>[4x]GSKLQICVEPTSQKLMPGSTLVLQCVAVGSPIPHYQWFKNELPLTHET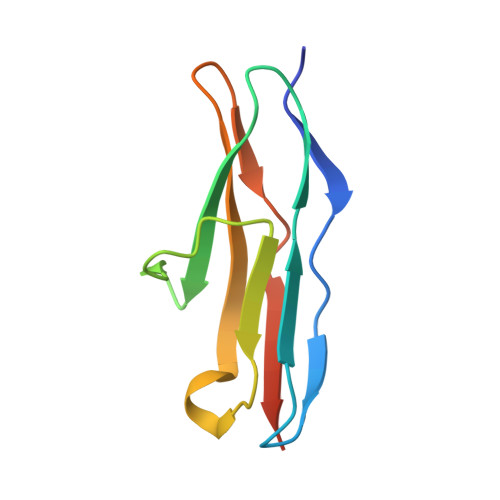KKLYMVPYVDLEHQGTYWCHVYNDRDSQDSKKVEIIIDELNNL>[2x]AGGG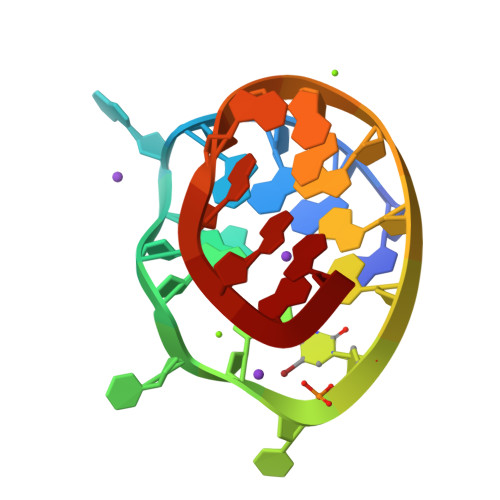AGGGCGCUGGGAGGAGGG> TVKIWVKYNEGFSNAVRKNV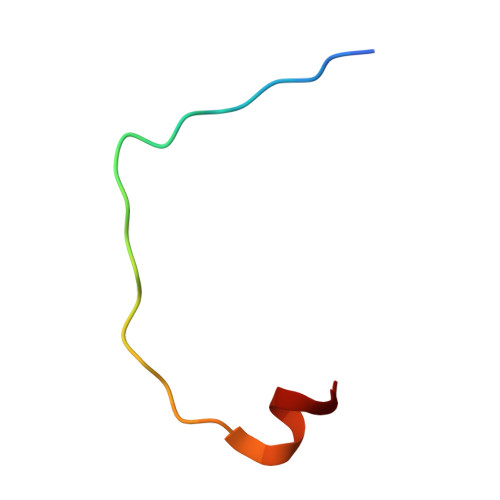TWNNLWE> MGSPASDPTVFHKRYLKKIRDLGEGHFGKVSLYCYDPTNDGTGEMVAVKALKADCGPQHRSGWKQEIDILRTLYHEHIIKYKGCCEDQGEKSLQLVMEYVPLGSLRDYLPRHSIGLAQLLLFAQQICEGMAYLHAQHYIHRNLAARNVLLDNDRLVKIGDFGLAKAVPEGHEYYRVREDGDSPVFWYAPECLKEYKFYYASDVWSFGVTLYELLTHCDSSQSPPTKFLEL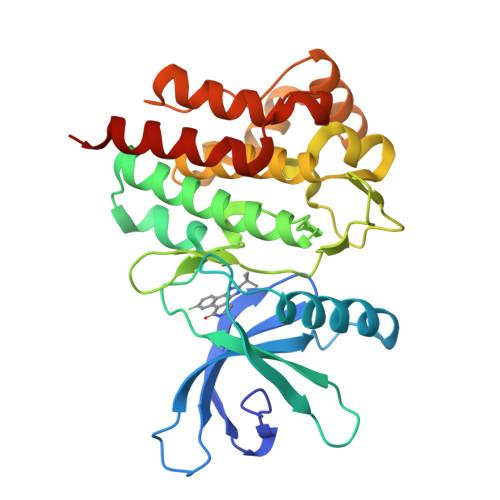IGIAQGQMTVLRLTELLERGERLPRPDKCPCEVYHLMKNCWETEASFRPTFENLIPILKTVHEKYRHHHHHH>[8x]CTAITLNGNSNYFGRNLDLDFSYGEEVIITPAEYEFKFRKEKAIKNHKSLIGVGIVANDYPLYFDAINEDGLGMAGLNFPGNAYYSDALENDKDNITPFEFIPWILGQCSDVNEARNLVEKINLINLSFSEQLPLAGLHWLIADREKSIVVEVTKSGVHIYDNPIGILTNNPEFNYQMYNLNKYRNLSISTPQ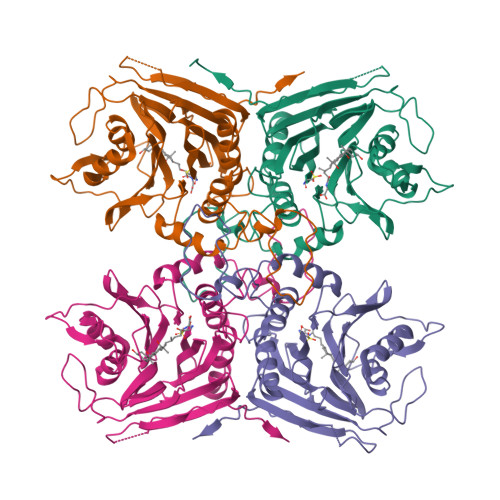NTFSDSVDLKVDGTGFGGIGLPGDVSPESRFVRATFSKLNSSKGMTVEEDITQFFHILGTVEQIKGVNKTESGKEEYTVYSNCYDLDNKTLYYTTYENRQIVAVTLNKDKDGNRLVTYPFERKQIINKLNLE> MTRGAWMCR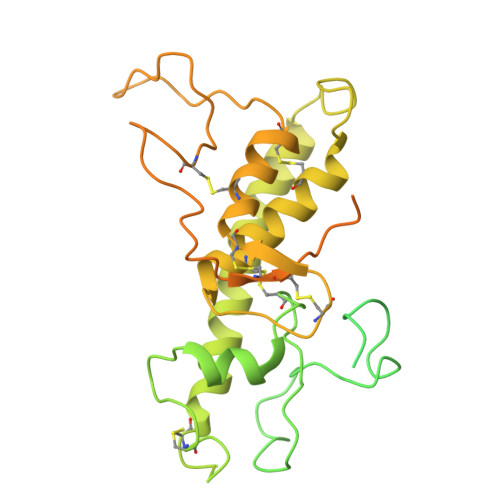QYDDGLKIWLAAPRENEKPFIDSERAQKWRLSLASLLFFTVLLSDHLWFCAEAKLTRARDKEHQQQQRQQQQQQQQQRQRQQQQQQRRQQEPSWPALLASMGESSPAAQAHRLLSASSSPTLPPSPGDGGGGGGKGNRGKDDRGKALFLGNSAKPVWRLETCYPQGASSGQCFTVENADAVCARNWSRGAAGGDGQEVRSKHPTPLWNLSDFYLSFCNSYTLWELFSGLSSPNTLNCSLDVVLKEGGEMTTCRQCVEAYQDYDHHAQEKYEEFESVLHKYLQSEEYSVKSCPEDCKIVYKAWLCSQYFEVTQFNCRKTIPCKQYCLEVQTRCPFILPDNDEVIYGGLSSFICTGLYETFLTNDEPECCDVRREEKSNNPSKGTVEKSGSCHRTSLTVSSATRLCNSRLKLCVLVLILLHTVLTASAAQNTAGLSFGGINTLEENSTNEELEDEVDAGSDYKDDDDKGSDYKDDDDK> GLPVMTTPGSTQFLTSDDFQSPSAMPQFDVTPEMQIPGRVNNLMEIAE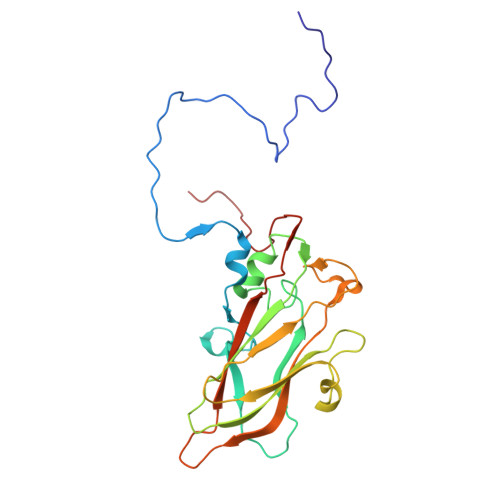VDSVVPVNNTDNNVNGLKAYQIPVQSNSDNRRQVFGFPLQPGANNVLNRTLLGEILNYYTHWSGSIKLTFMFCGSAMATGKFLLAYSPPGAGVPKNRRDAMLGTHVIWDVGLQSSCVLCVPWISQTHYRYVVEDEYTAAGYVTCWYQTNIIVPADVQSTCDILCFVSACNDFSVRMLKDTPFIRQDNFYQ> MKDQLSDEQKETILKALNDAIEKGPWDKSNFLRVIGKKLIAIRDRF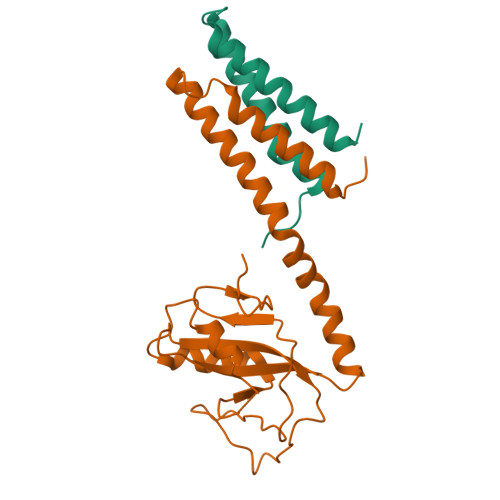LKRIGAASQAQLQAESHLANQIALQSGQQEIYVSLYSSDGSNLQSWEKIVGSLPRQMISRPIYADEEDIKAILKTKENKQNEAYVAIYISQSDILHLSADKAPVDKLGKPLLTLKDKSISLENISRFVHVSGVYRYSNGRLIKNA;> MGNNTDDSARNPFGFYTPPRVKEIGEPDVTDATLGSVYSEIISPVKDCILTVAKAVSFNPGGKDNTDAVEVLTELNTKVERAALNQPILTTKTERMFGAAESEKSSEPPSHDERGFKLSS> GPGYQDPLSIDERLQA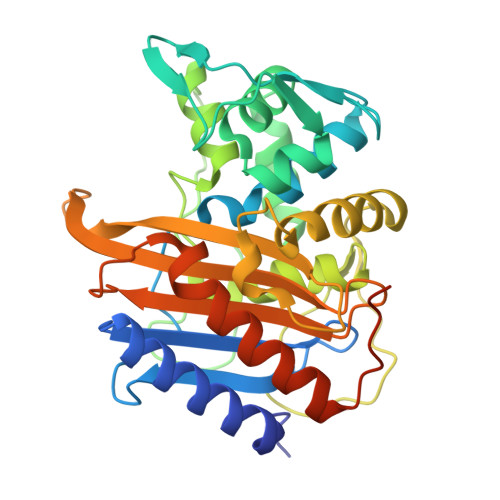LVYRELNNAVAFNKAESGSAVLVDVNTGEVLAMANSPGRNRTITDVFEPGSTVKPMVVMTALQRGVVRENSVLNTIPYRINGHEIKDVARYSELTLTGVLQKSSNVGVSKLALAMPSSALVDTYSRFGLGKATNLGLVGERSGLYPQKQRWSDIERATFSFGYGLMVTPLQLARVYATIGSYGIYRPLSITKVDPPVPGERVFPESIVRTVVHMMESVALPGGGGVKAAIKGYRIAIKTGTAKKVGPDGRYINKYIAYTAGVAPASQPRFALVVVINDPQAGKYYGGAVSAPVFGAIMGGVLRTMNIEPDALTTGDKNEFVINQGEGTGGRS> MYESILSIKPYNLSKEQITWVNQTLVSLSDDEKLGQLICEIIWDKPGCDPLDVMKHFLPGAVMYRPFKAKRMREFTQRLQKASKIPLLIACNLERGGSGG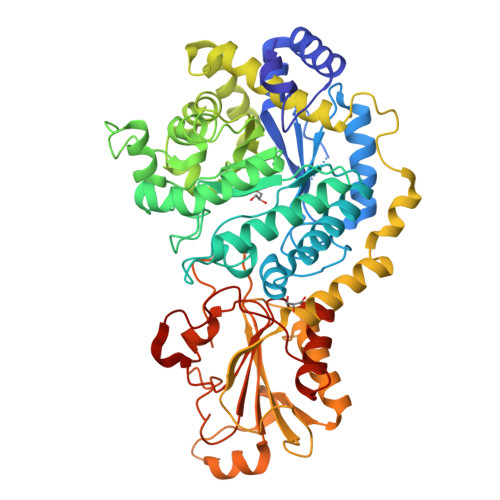NGGMEDGTYVASPMGVAATDDESSAEHLGEVCASEGSAVGVNWTYEPIIDIDMNPENPITNVRTYGSDPERIIRMAKAYCRGCRKWGVLTTIKHFPGDGVDYRDQHLMSSVNNLSADEWMDTYGRIYQALIEDGAETLMSAHIRQPNVTRMVNPLIKDEEIMPGSLSKELMQGILRGRFHFNGLICTDATQMVGYTCSMPRHEALPTSIQNGADMLTFTLNPTEDFKALQEGLSCGLLTHERLDEAVARILGMKAKLRLPERKDVVPPLHAMERIQSKKHKKWALEIADESITLVKDKQKGLLPLSPQKTKRIILVQATNEKPEGGYLSEARLFKGLLEKEGFIVHWFEEVPRPGTGYSIEDLKRDTDLFIYYANFKVSSNQTTIRLVWSDFLGDSSPKFVCDVPTLFLSFSNPYHLVDVPMVKTYINAYTSNEATVRMMIEKLMGRSSFKGKSPVDPFAGLWDARLHHHHHH> CSALIKLLPGGHDLLVAHNTWNSYQNMLRIIKKYRLQFR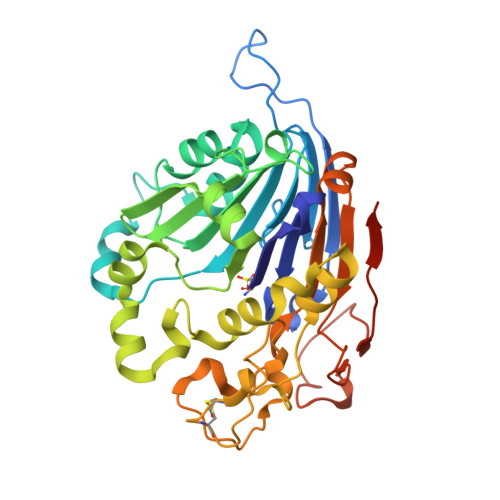EGPQEEYPLVAGNNLVFSSYPGTIFSGDDFYILGSGLVTLETTIGNKNPALWKYVQPQGCVLEWIRNVVANRLALDGATWADVFKRFNSGTYNNQWMIVDYKAFLPNGPSPGSRVLTILEQIPGMVVVADKTAELYKTTYWASYNIPYFETVFNASGLQALVAQYGDWFSYTKNPRAKIFQRDQSLVEDMDAMVRLMRYNDFLHDPLSLCEACNPKPNAENAISARSDLNPANGSYPFQALHQRAHGGIDVKVTSFTLAKYMSMLAASGPTWDQCPPFQWSKSPFHSMLHMGQPDLWMFSPIRVPWDGRGSHHHHHHG> DDEATILADNKCMCTRVTSRIIPSTEDPNEDIVERNIRIVVPLNNRENISDPTSPLRRNFVYHLSDVCKKCDPVEVELEDQVVTAT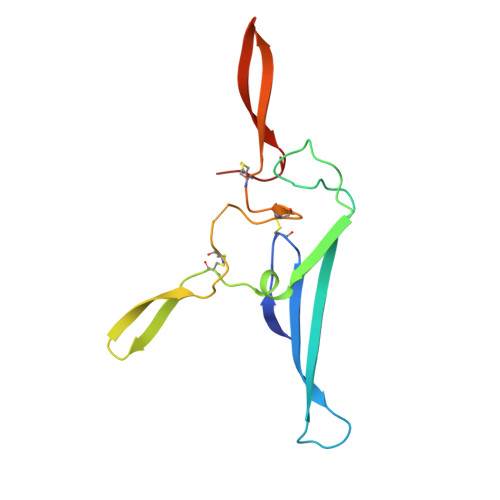QSNICNEDDGVPETCYMYDRNKCYTTMVPLRYHGETKMVQAALTPDSCYPD>ALVAEDAPVLSKAFVDRVNRLNRGIWKAKYDGVMQNITLREAKRLNGVIKKNNNASILPKRRFTEEEARAPLPSSFDSAEAWPNCPTIPQIADQSACGSCWAVAAASAMSDRFCTMGGVQDVHISAGDLLACCSDCGDGCNGGDPDRAWAYFSSTGLVSDYCQPYPFPHCSHHSKSKNGYPPCSQFNFDTPKCDYTCDDPTIPVVNYRSWTSYALQGEDDYMRELFFRGPFEVAFDVYEDFIAYNSGVYHHVSGQYLGGHAVRLVGWGTSNGVPYWKIANSWNTEWGMDGYFLIRRGSSECGIEDGGSAGIPLAPNTAHHHHHHH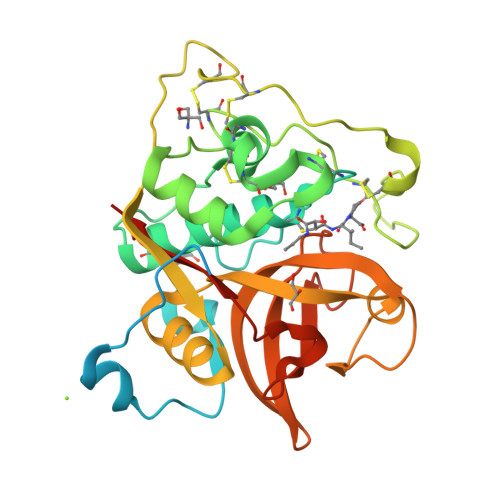[2x]> DIVQHMEDIGGAPPVSCVTNEILGVTCAPQ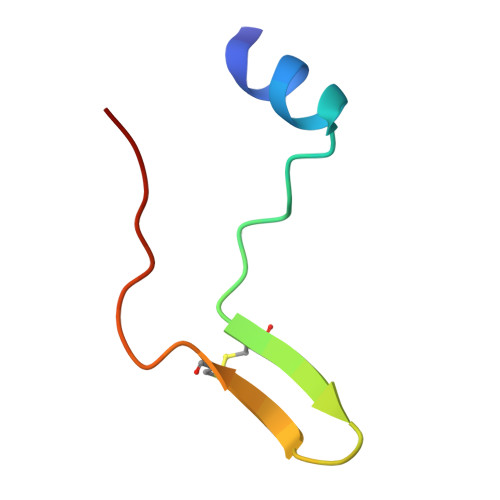AIAKATT> ADGKSTRYWDCCKPSCGWAKKAPVNQPVFSCNANFQRLTDFDAKSGCEPGGVAYSCADQTPWAVNDDFAFGFAATSIAGSNEAGWCCACYELTFTSGPVAGKKMVVQSTSTGGDLGSNHFDLNIPGGGVGIFDGCTPQFGGLPGQRYGGISSRNECDRFPDALKPGCY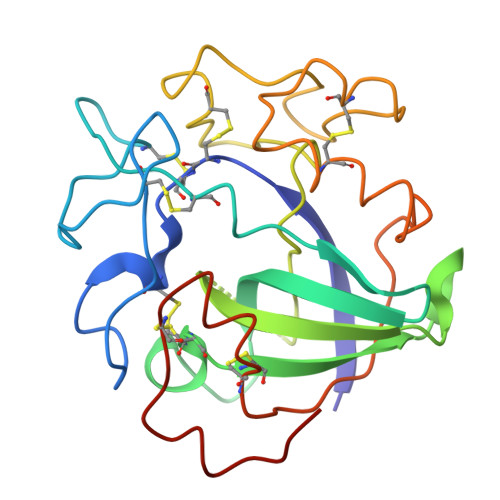WRFDWFKNADNPSFSFRQVQCPAELVARTGCRRNDDGNFPAVQIP> ALWQFNGMIKCKIPSSEPLLDFNNYGCYCGLGGSGTPVDDLDRCCQTHENCYKQAKKL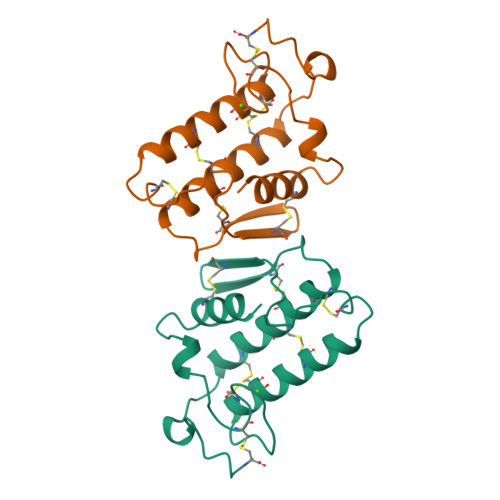DSCKVLVDNPYTNNYSYSCSNNEITCSSENNACEAFICNCDRNAAICFSKVPYNKEHKNLDKKNC N-(2-ISOPROPYLPHENYL)-3-[(2-THIENYLMETHYL)THIO]-1H-1,2,4-TRIAZOL-5-AMINE | C16 H18 N4 S2 | 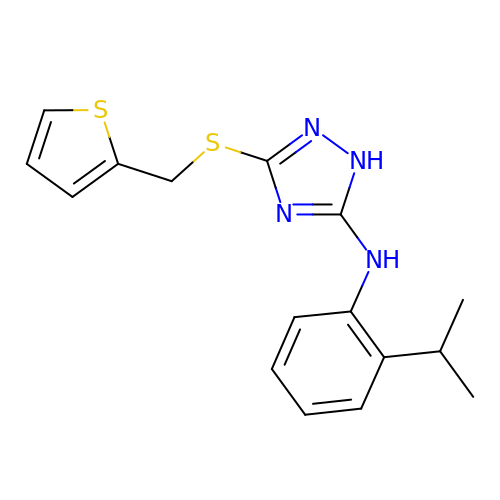QMNSHLAPQLBIGP-UHFFFAOYSA-N>[2x]MVKLKNVTKTYKMGEEIIYALKNVNLNIKEGEFVSIMGPSGSGKSTMLNIIGCLDKPTEGEVYIDNIKTNDLDDDELTKIRRDKIGFVFQQFN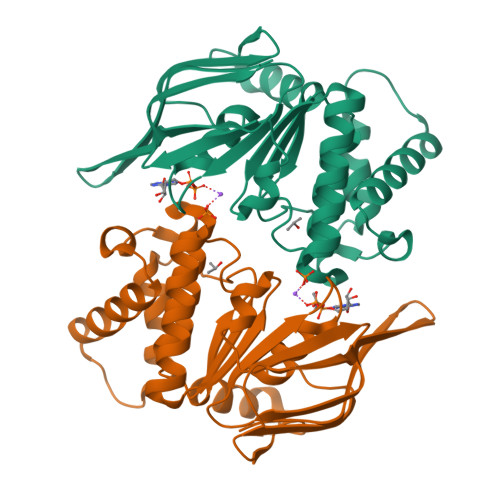LIPLLTALENVELPLIFKYRGAMSGEERRKRALECLKMAELEERFANHKPNQLSGGQQQRVAIARALANNPPIILADQPTWALDSKTGEKIMQLLKKLNEEDGKTVVVVTHDINVARFGERIIYLKDGEVEREEKLRGFDDR> STQLDIVIVLDGSNSIYPWDSVTAFLNDLLERMDIGPKQTQVGIVQYGENVTHEFNLNKYSSTEEVLVAAKKIVQRGGRQTMTALGTDTARKEAFTEARGARRGVKKVMVIVTDGESHDNHRLKKVIQDCEDENIQRFSIAILGSYNRGNLSTEKFVEEIKSIASEPTEKHFFNVSDEIALVTIVKTLGERI;> STQLDIVIVLDGSNSIYPWDSVTAFLNDLLERMDIGPKQTQVGIVQYGENVTHEFNLNKYSSTEEVLVAAKKIVQRGGRQTMTALGIDTARKEAFTEARGARRGVKKVMVIVTDGESHDNHRLKKVIQDCEDENIQRFSIAILGSYNRGNLSTEKFVEEIKSI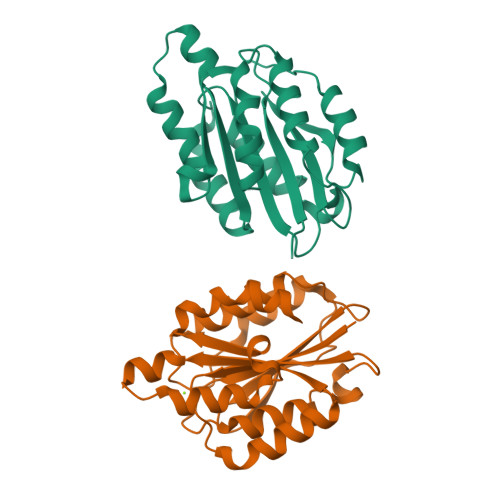ASEPTEKHFFNVSDEIALVTIVKTLGERI> GSHMASMTGGQQMGRGSMEEF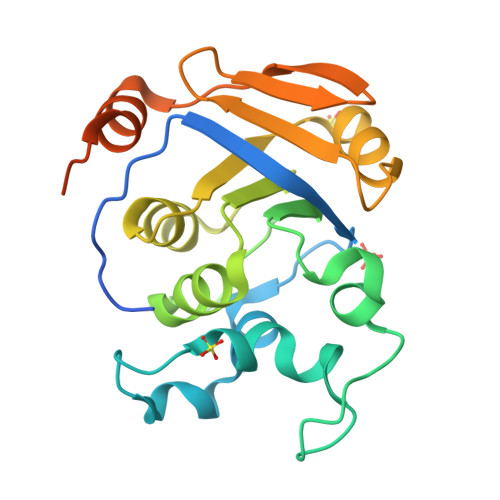TIYTGTTVPLMNDNIDTDQILPKQFLKLIDKKGFGKYLMYEWRYLDNNYTENPDFIFNQPEYREASILITGDNFGAGSSREHAAWALADYGFKVIVAGSFGDIHYNNDLNNGILPIIQPKEVRDKLAKLKPTDEVTVNLFEQKIYSPVGDFSFDIDGEWKHKLLNGLDDIGITLQYEDLIAQYEQNRPSYWH In Escherichia coli, cytotoxic DNA methyl lesions on the N1 position of purines and N3 position of pyrimidines are primarily repaired by the 2-oxoglutarate (2-OG) iron(II) dependent dioxygenase, AlkB. AlkB is a member of the iron(II) dependent 2-oxoglutarate (2-OG) dioxygenase superfamily that couples decarboxylation of 2-OG to succinate to oxidation of methylation damage primarily in the form of 1-methyladenine (1-meA) and 3-methylcytosine (3-meC) upon binding of dioxygen to the iron(II) cofactor. The AlkB enzyme recognizes and repairs other alkylated DNA lesions such as 3-methylthymine (3-meT), 1-methylguanine (1-meG), and 1,N6-ethenoadenine (εA), albeit with lower efficiency. AlkB repairs methylated DNA damage in ssDNA much more efficiently than in duplex DNA and displays significantly different activity on structurally similar methylated bases.

We determined the structure of the full length E. coli AlkB protein in complex with a 17-mer ssDNA oligonucleotide containing a 1-meG lesion to 2.2 Å resolution and the structure of the AlkB holoenzyme in the absence of nucleotide substrate to 2.9 Å resolution. The structure of the ssDNA complex was determined using a D135A mutation of AlkB because our mutagenesis data revealed that this residue is responsible for the specificity of 1-meA and 3-meC lesions. Our DNA binding experiments further showed this mutant has a higher affinity for DNA that allowed us to crystallize the DNA complex without the need for cross-linking as was done for the dsDNA complex. Interestingly, in the crystals of the AlkB-ssDNA complex two monomers crystallized in the asymmetric unit, but only one monomer was bound to DNA. Of the 17 nucleotides present in the ssDNA oligonucleotide, only 12 were able to be modeled into the electron density of the structure. The phosphodiester backbone of the ssDNA binds in an electropositive DNA binding groove that is created by a T51-Y55 DNA binding loop, S129, and K127. The substrate base is bound in the active site pocket formed by hydrophobic stacking interaction of W69 and H131. The methyl group of the 1-meG is adjacent to the bound metal ion and properly positioned for oxidative repair. The O6 oxygen of the methylated guanine is pointed towards the space created by the absence of a carboxylate side chain in the D135A mutation supporting the idea that residue D135 provides selectivity for binding adenine and cytosine bases in the active site. Additionally, with DNA bound and a substrate base in the active site, the Y76 side chain rotates to close the active site pocket.

>GPHMLDLFADAEPWQEPLAAGAVILRRFAFNAAEQLIRDINDVASQSPFRQMVTPGGYTMSVAMTNCGHLGWTTHRQGYLYSPIDPQTNKPWPAMPQSFHNLCQRAATAAGYPDFQPDACLINRYAPGAKLSLHQDKAEPDLRAPIVSVSLGLPAIFQFGGLKRNDPLKRLLLEHGDVVVWGGESRLFYHGIQPLKAGFHPLTIDCRYNLTFRQAGKKE[2x]> RTIRYVRYESELQMPDIMRLITKDLSEPYSIYTYRYFIHNWPQLCFLAMVGEECVGAIVCKLDMHKKMFRRGYIAMLAVDSKYRRNGIGTNLVKKAIYAMVEGDCDEVVLETEITNKSALKLYENLGFVRDKRLFRYYLNGVDALRLKLWLR;> MVMKASVDDDDSGWELSMPEKMEKSNTNWVDITQDFEEACRELKLGELLHDKLFGLFEAMSAIEMMDPKMDAGMIGNQVNRKVLNFEQAIKDGTIKIKDLTLPELIGIMDTCFCCLITWLEGHSLAQTVFTCLYIHNPDFIEDPAMKAFALGILKICDIAREKVNKAAVFEEEDFQSMTYGFKMANSVTDLRVTGMLKDVEDDMQRRVKSTRSRQGEERDPEVELEHQQCLAVFSRVKFTRVLLTVLIAFTK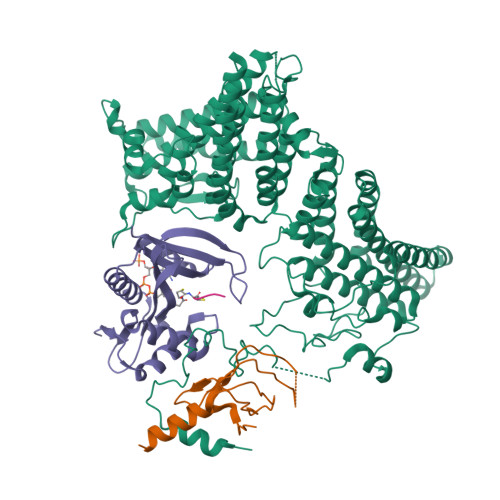KETSAVAEAQKLMVQAADLLSAIHNSLHHGIQAQNDTTKGDHPIMMGFEPLVNQRLLPPTFPRYAKIIKREEMVNYFARLIDRIKTVCEVVNLTNLHCILDFFCEFSEQSPCVLSRSLLQTTFLVDNKKVFGTHLMQDMVKDALRSFVSPPVLSPKCYLYNNHQAKDCIDSFVTHCVRPFCSLIQIHGHNRARQRDKLGHILEEFATLQDEAEKVDAALHTMLLKQEPQRQHLACLGTWVLYHNLRIMIQYLLSGFELELYSMHEYYYIYWYLSEFLYAWLMSTLSRADGSQMAEERIMEEQQKGRSSKKTKKKKKVRPLSREITMSQAYQNMCAGMFKTMVAFDMDGKVRKPKFELDSEQVRYEHRFAPFNSVMTPPPVHYLQFKEMSDLNKYSPPPQSPELYVAASKHFQQAKMILENIPNPDHEVNRILKVAKPNFVVMKLLAGGHKKESKVPPEFDFSAHKYFPVVKLV;> MAGAGPTMLLREENGCCSRRQSSSSAGDSDGEREDSAAERARQQLEALLNKTMRIRMTDGRTLVGCFLCTDRDCNVILGSAQEFLKPSDSFSAGEPRVLGLAMVPGHHIVSIEVQRESLTGPPYL;> MLGP>[6x]MIYPDEAMLYAPVEWHDCSEGFEDIRYEKSTDGIAKITINRPQVRNAFRPLTVKEMIQALADARYDDNIGVIILTGAGDKAFCSGGDQKVRGDYG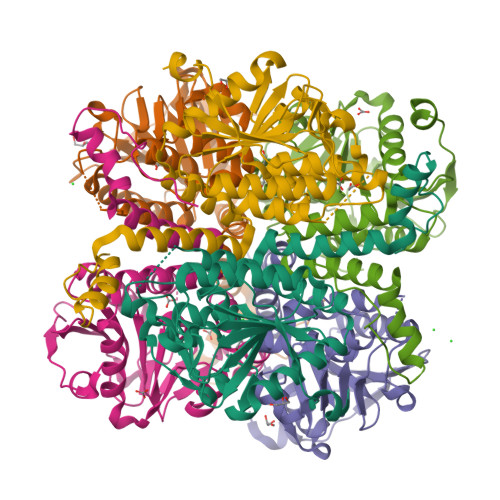GYKDDSGVHHLNVLDFQRQIRTCPKPVVAMVAGYSIGGGHVLHMMCDLTIAADNAIFGQTGPKVGSFDGGWGASYMARIVGQKKAREIWFLCRQYDAKQALDMGLVNTVVPLADLEKETVRWCREMLQNSPMALRCLKAALNADCDGQAGLQELAGNATMLFYMTEEGQEGRNAFNQKRQPDFSKFKRNP>[2x]MASLTVKAYLLGKEDAAREIRRFSFSFSPEPEAEAEAAAGPGPCERLLSRVAALFPALRPGGFQAHYRAERGDLVAFSSDEELTMA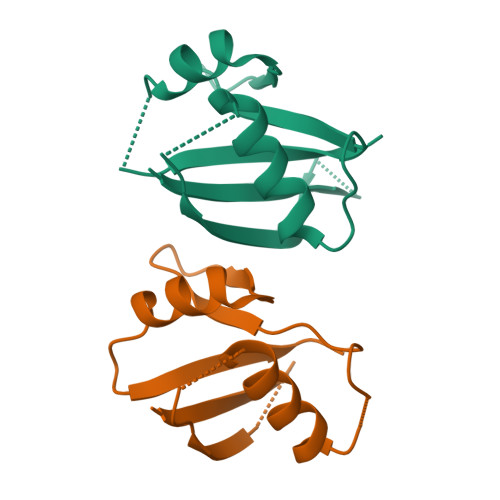MSYVKDDIFRIYIKEK;>[2x]MASLTVKAYLLGKEDAAREIARFSFSFSPEPEAEAEAAAGPGPCERLLSRVAALFPALRPGGFQAHYRDEDGDLVAFSSDEELTMAMSYVKDDIFRIYIKEK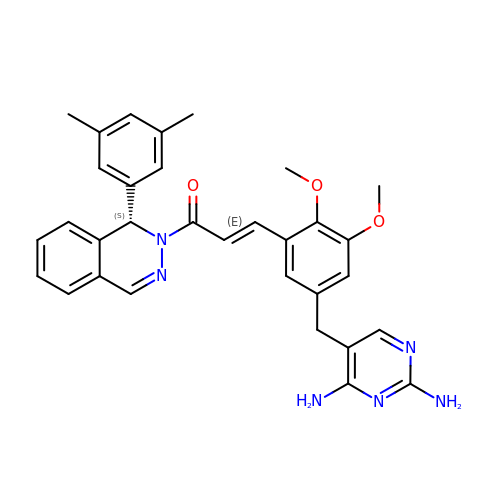(2E)-3-{5-[(2,4-diaminopyrimidin-5-yl)methyl]-2,3-dimethoxyphenyl}-1-[(1S)-1-(3,5-dimethylphenyl)phthalazin-2(1H)-yl]prop-2-en-1-one | C32 H32 N6 O3 | YJNMFIWPSJEFDR-MOGHOSLNSA-N> MDNLLRHLKISKEQITPVVLVVGDPGRVDKIKVVCDSYVDLAYNREYKSVECHYKGQKFLCVSHGVGSAGCAVCFEELCQNGAKVIIRAGSCGSLQPDLIKRGDICICNAAVREDRVSHLLIHGDFPAVGDFDVYDTLNKCAQELNVPVFNGISVSSDMYYPNKIIPSRLEDYSKANAAVVEMELATLMVIGTLRKVKTGGILIVDGCPFKWDEGDFDNNLVPHQLENMIKIALGACAKLATKYAAHHHHHH

Purines are obtained by the parasite from the host erythrocyte mostly via hypoxanthine, the major purine base salvaged by Plasmodium, through metabolizing adenosine via the sequential action of adenosine deaminase and purine nucleoside phosphorylase (PfPNP). PfPNP catalyzes the phosphorylation of inosine and guanosine to ribose-1 phosphate and hypoxanthine or guanine, respectively. Since hypoxanthine synthesized through this purine salvage pathway constitutes a major source of purines for the parasite, PfPNP is essential for parasite survival. Like in previously reported structures, PfPNP forms a homo-hexamer, with three 2-fold symmetrical dimers arranged around a crystallographic three-fold symmetry axis running through the central aperture of the assembly.

To understand the mode of inhibition at the atomic level, we co-crystallized PfPNP with MMV000848 and determined the structure of this complex at 1.85 Å in space group R32, which is isomorphous to the structures of PfPNP bound to quinine and mefloquine reported earlier. The MMV000848 inhibitor (MW = 308.4 Da, 1-carbazol-9-yl-3-cyclopentylamino-propan-2-ol) is composed of one heterocyclic carbazole aromatic group of three fused rings connected to a cyclopentyl-amino five-carbon ring by a propane moiety that comprises a hydroxyl group at position 2. The latter forms a hydrogen bond with Asp206, and several water-mediated contacts with Ser91, Asp206 and the hydroxyl group of Tyr160. Thus, the conserved active site residue Asp206 appears key for the stabilization of MMV00848 in the active site pocket. The fused aromatic rings of the carbazole group of MMV000848 fits snugly in the inosine-binding region where it forms an edge-to-face π-π interactions with the Tyr160 phenyl ring and CH-π interactions with Val181 side chain. Although It does not form direct contacts with MMV000848, the bound phosphate ion plays a key role in stabilizing the complex: it forms hydrogen bonds with Ser91 and Arg88, bifurcated hydrogen bonds with Arg45′ from the other monomer (residues form the monomer partner in the dimer are labeled with a prime) and a water-mediated hydrogen bond with Glu184. A conspicuous difference is observed in the active site loop that joins residues Trp212 to Val222 of the enzyme. While this loop is ordered in the complex with transition state analogs such as ImmH where it folds into helix ɑ8, here it is disordered in the complex with MMV000848.> ENALKKSDGTRKSRITNYPKLEDANKAGTKEGYKCTLVLTEGDSALSLAVAGLAVVGRDYYGCYPLRGKMLNVREASADQILKNAEIQAIKKIMGLQHRKKYEDTKSLRYGHLMIMTDQDHDGSHIKGLIINFLESSFLGLLDIQGFLLEFITPIIKVSITKPTKNTIAFYNMPDYEKWREEESHKFTWKQKYYKGLGTSLAQEVREYFSNLDRHL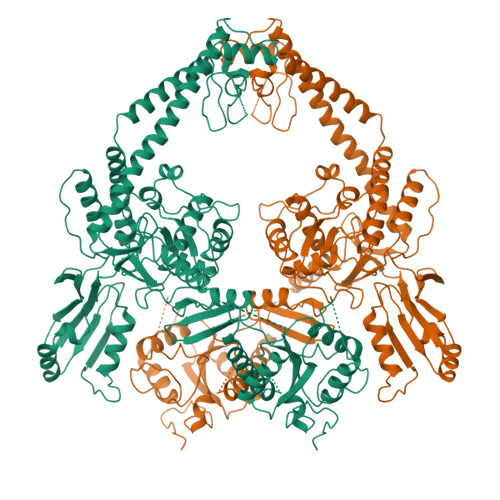KIFHSLQGNDKDYIDLAFSKKKADDRKEWLRQYEPGTVLDPTLKEIPISDFINKELILFSLADNIRSIPNVLDGFKPGQRKVLYGCFKKNLKSELKVAQLAPYVSECTAYHHGEQSLAQTIIGLAQNFVGSNNIYLLLPNGAFGTRATGGKDAAAARYIYTELNKLTRKIFHPADDPLYKYIQEDEKTVEPEWYLPILPMILVNGAEGIGTGWSTYIPPFNPLEIIKNIRHLMNDEELEQMHPWFRGWTGTIEEIEPLRYRMYGRIEQIGDNVLEITELPARTWTSTIKEYLLLGLSGNDKIKPWIKDMEEQHDDNIKFIITLSPEEMAKTRKIGFYERFKLISPISLMNMVAFDPHGKIKKYNSVNEILSEFYYVRLEYYQKRKDHMSERLQWEVEKYSFQVKFIKMIIEKELTVTNKPRNAIIQELENLGFPRFNKEGKPYYGSPNDEIAEQINDVKGATSDEEDEESSHEDTENVINGPEELYGTYEYLLGMRIWSLTKERYQKLLKQKQEKETELENLLKLSAKDIWNTDLKAFEVGYQEFLQRDAEARGGNVPNKGSKTKGKGKRKLVDDED>[2x]NKGTDDATADSRKTYTLTDYLKNTYRLKLYSLRWISDHEYLYKQENNILVFNAEYGNSSVFLENSTFDEFGHSINDYSISPDGQFILLEYNYVKQWRHSYTASYDIYDLNKRQLITEERIPNNTQWVTWSPVGHKLAYVWNNDIYVKIEPNLPSYRITWTGKEDIIYNGITDWVYEEEVFSAYS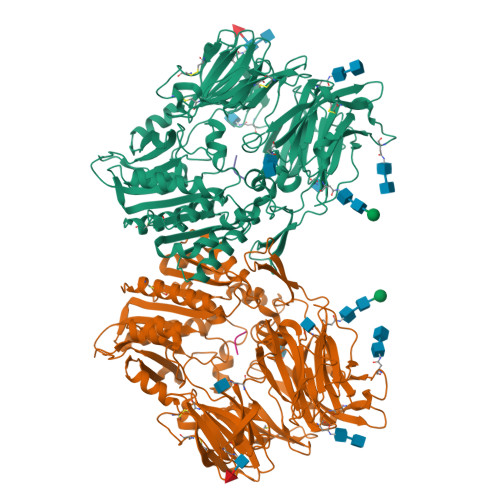ALWWSPNGTFLAYAQFNDTEVPLIEYSFYSDESLQYPKTVRVPYPKAGAVNPTVKFFVVNTDSLSSVTNATSIQITAPASMLIGDHYLCDVTWATQERISLQWLRRIQNYSVMDICDYDESSGRWNCLVARQHIEMSTTGWVGRFRPSEPHFTLDGNSFYKIISNEEGYRHICYFQIDKKDCTFITKGTWEVIGIEALTSDYLYYISNEYKGMPGGRNLYKIQLSDYTKVTCLSCELNPERCQYYSVSFSKEAKYYQLRCSGPGLPLYTLHSSVNDKGLRVLEDNSALDKMLQNVQMPSKKLDFIILNETKFWYQMILPPHFDKSKKYPLLLDVYAGPCSQKADTVFRLNWATYLASTENIIVASFDGRGSGYQGDKIMHAINRRLGTFEVEDQIEAARQFSKMGFVDNKRIAIWGWSYGGYVTSMVLGSGSGVFKCGIAVAPVSRWEYYDSVYTERYMGLPTPEDNLDHYRNSTVMSRAENFKQVEYLLIHGTADDNVHFQQSAQISKALVDVGVDFQAMWYTDEDHGIASSTAHQHIYTHMSHFIKQCFSLP;>[2x]MDPVDPNIE(benzyloxy)acetic acid 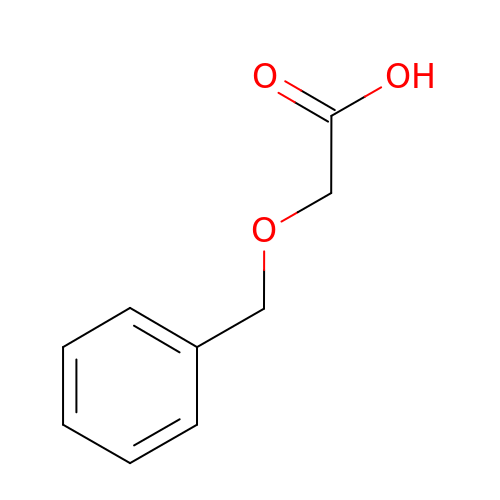| C9 H10 O3 | GRZHHTYDZVRPIC-UHFFFAOYSA-N>[6x]EEGQKVDHCARHGEKLLLFCQEDSKVICWLCERSQEHRGHHTFLMEEVAQEYHVKLQTALEMLRQKQQEAETERNQVAKRVPKAPPEEKEALIARGKALGEQTQYMR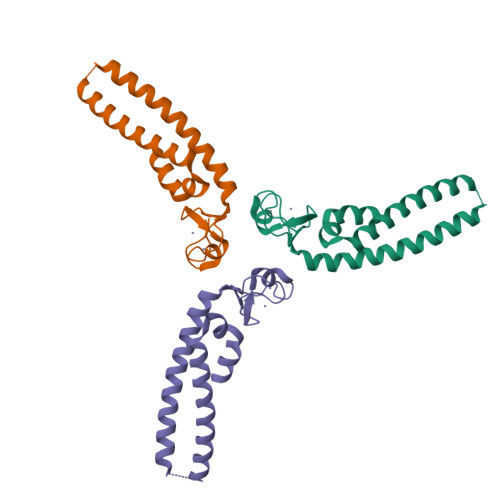ELISELEHRLQGSMMDLLQGVDGIIKRIENMTLK> MANAASGMAVHDDCKLRFLELKAKRTHRFIVYKIEEKQKQVVVEKVGQPIQTYE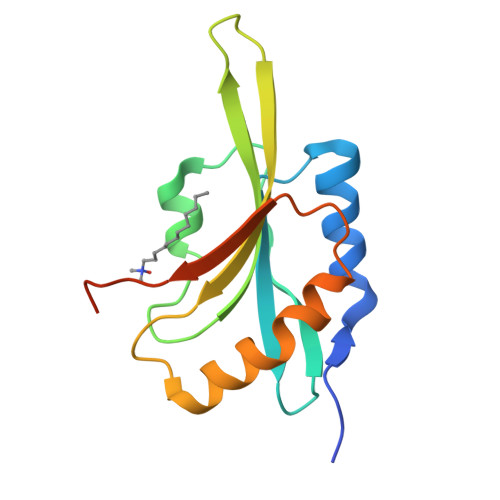EFAACLPADECRYAIYDFDFVTAENCQKSKIFFIAWCPDIAKVRSKMIYASSKDRFKRELDGIQVELQATDPTEMDLDVFRSRAN> MTLSILVAHDLQRVIGFENQLPWHLPNDLKHVKKLSTGHTLVMGRKTFESIGKPLPNRRNVVLTSDTSFNVEGVDVIHSIEDIYQLPGHVFIFGGQTLFEEMIDKVDDMYITVIEGKFRGDTFFPPYTFED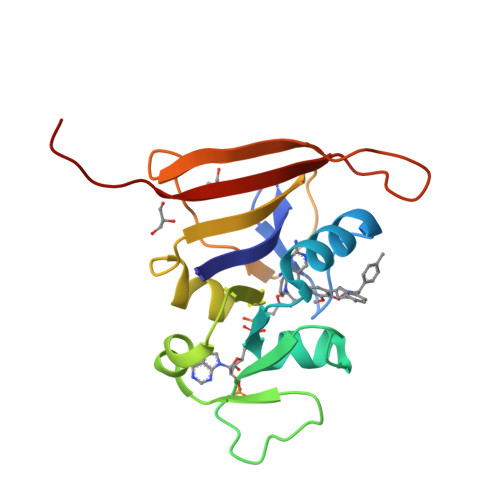WEVASSVEGKLDEKNTIPHTFLHLIRKKLVPR>[2x]MQTKLTIWCSEKQVDILQKLGEEFKAKYGIPVEVQYVDFGSIKSKFLTAAPQGQGADIIVGAHDWVGELAVNGLIEPIPNFSDLKNFYDTALKAFSYGGKLYGVPYAMEAVALIYNKDYVDSVPKTMDELIEKAKQIDEEYGGEVRGFIYDVANFYFSAPF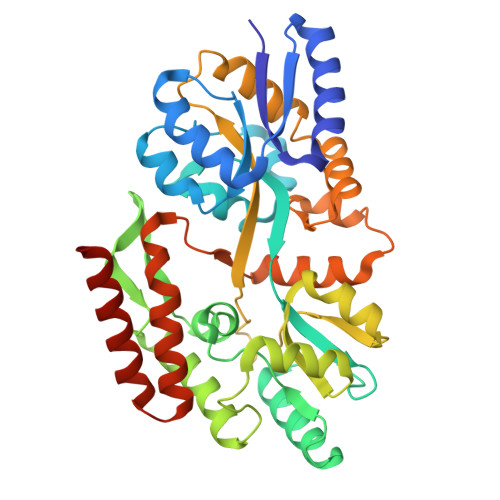ILGYGGYVFKETPQGLDVTDIGLANEGAVKGAKLIKRMIDEGVLTPGDNYGTMDSMFKEGLAAMIINGLWAIKSYKDAGINYGVAPIPELEPGVPAKPFVGVQGFMINAKSPNKVIAMEFLTNFIARKETMYKIYLADPRLPARKDVLELVKDNPDVVAFTQSASMGTPMPNVPEMAPVWSAMGDALSIIINGQASVEDALKEAVEKIKAQIEKGSHHHHHH> MASMKKKGSVVIVGRINLSGDTAYAQQTRGEEGCQETSQTGRDKNQVEGEVQIVSTATQTFLATSINGVLWTVYHGAGTRTIASPKGPV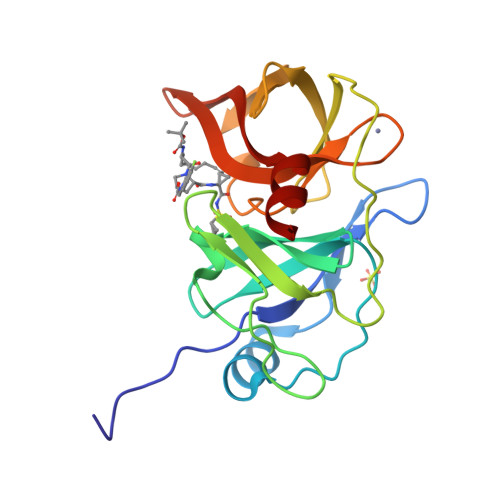TQMYTNVDKDLVGWQAPQGSRSLTPCTCGSSDLYLVTRHADVIPVRRRGDSRGSLLSPRPISYLKGSAGGPLLCPAGHAVGIFKAAVSTRGVAKAVDFIPVESLETTMR> PVPTGVSFDYIVVGGGAGGIPAADKLSEAGKSVLLIEKGFASTANTGGTLGPEWLEGHDLTRFDVPGLCNQIWVDSKGIACEDTDQMAGCVLGGGTAVNAGLWFKPYSLDWDYLFPDGWKYNDVQPAINRALSRIPGTDAPSTDGKRYYQEGFEVLSKGLAAGGWTSVTANNAPDKKNRTFAHAPFMFAGGERNGPLGTYFQTAKKRNNFDVWLNTSVKRVIREGGHITGVEVEPFRDGGYEGIVPVTKVTGRVILSAGTFGSAKILLRSGIGPEDQLEVVAASEKDGPTMIGNSSWINLPVGYNLDDHLNTDTVISHPDVVFYDFYEAWDDPIESDKNSYLESRTGILAQAAPNIGPMFWEEIVGADGIVRQLQWTARVEGSLGAPNGHTMTMSQYLGRGATSRGRMTITPSLTTIVSDVPYLKDPNDKEAVIQGIINLQNALQNVANLTWLFPNSTITPREYVESMVVSPSNRRSNHWMGTNKLGTDDGRKGGSAVVDLDTRVYGTDNLFVIDASIFPGVPTTNPTSYIVVAAEHASSRILALPDLEPVPKYGQCGGREWTGSFVCADGSTCEYQNEWYSQCL

An oxidative system was recently discovered in which extracellular flavocytochromes, that is, cellobiose dehydrogenases (CDHs), cooperate with copper-dependent lytic polysaccharide monooxygenases (LPMOs)8910111213 to catalyse redox-mediated glycosidic bond cleavage in crystalline cellulose, hemicelluloses and starch. CDHs are large flavocytochromes containing a haem b-binding cytochrome domain (CYT) connected by a long, flexible linker to a flavin adenine dinucleotide (FAD)-binding dehydrogenase domain (DH). The DH domain oxidizes cellobiose at the C1 position to cellobiono-1,5-lactone with reduction of FAD. The ensuing step involves inter-domain electron transfer (IET) from the reduced FAD to CYT haem b, presumably by single electron-transfer (ET) events, followed by ET from CYT to external electron acceptors such as LPMOs.

The active site of CDH has two glucosyl-binding subsites for cellobiose binding, subsite B (for binding site) and C (for catalytic site). Superimposition of the structures of MtCDH and MtDH-CBLM with ligand-free MtDH revealed that only two active-site side chains differ in conformation: the indole ring of Trp295 tilts slightly ‘upwards' with a maximum ring displacement of 1.4 Å, and Arg601 undergoes a conformational change involving 180° rotations of χ3 and χ4 on ligand binding at site B.>SLEIPSKQIDYRDVFIEFLTTFKGNNNQNKYIERINELVAYRKKSLIIEFSDVLSFNENLAYEIINNTKIILPILEGALYDHILQLDPTYQRDIEKVHVRIVGIPRVIELRKIRSTDIGKLITIDGILVKVTPVKERIYKATYKHIHPDCMQEFEWPEDEEMPEVLEMPTICPKCGKPGQFRLIPEKTKLIDWQKAVIQERPEEVPSGQLPRQLEIILEDDLVDSARPGDRVKVTGILDIKQDSPVKRGSRAVFDIYMKVSSIEVSGGSGGSSEEDEKKIKDLAKDPWIRDRIISSIAPSIYGHWELKEALALALFGGVPKVLEDTRIRGDIHILIIGDPGTAKSQMLQFISRVAPRAVYTTGKGSTAAGLTAAVVREKGTGEYYLEAGALVLADGGIAVIDEIDKMRDEDRVAIHEAMEQQTVSIAKAGIVAKLNARAAVIAAGNPKFGRYISERPVSDNINLPPTILSRFDLIFILKDQPGEQDRELANYILDVHSGKSTKNIIDIDTLRKYIA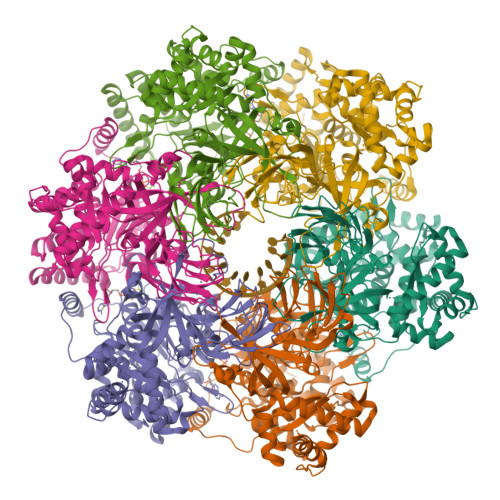YARKYVTPKITSEAKNLITDFFVEMRKKSSETPDSPILITPRQLEALIRISEAYAKMALKAEVTREDAERAINIMRLFLESVGVDMESGKIDID[6x]> MLDDNRPMDFAKDKNSATLWAKKRKQVWLNNLSKAESTSINNYIKNSSEINSYSIKKKFALDNYEGIETLNEDLKNISTAVKKSMLTKPLYVYYYEANDKFGFNQNLESSLDSNIIDEEAINNFAKKISDTNFIQDGFKDVTMTEPDINSKLPILVHLKLPTNTPAASYGNDEENLRVLIDQGYSLKATGLSIVTIKGKQYAKVDADLIKQLNFENDVISASQWGEENYAPWLKELTSNELRDINNYLGGGYTAINKYLLDGTIGENTSKEDLEEKISNISSALKKRKIPEDIITYRRMGPNEFGLDLNSPDYDFNKVENVSKFKEKWLGKTIPVKTFISTTVLSNNISAFAKRKLILRL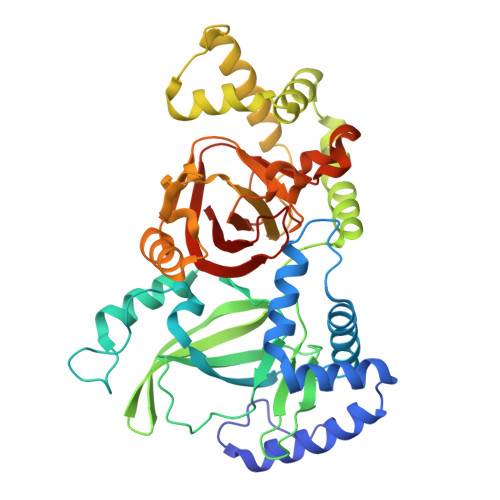HLPNGSNAAYVSVAEGYKNEYEVLIDHGYSYKIDNITEYYDESSLGGKTNKLIIDATLI>[6x]GMNKPCIISVAITGSLPRKKDNPAVPITVSEQVESTQAAFEAGATLVHLHVRNDDETPTSNPDRFALVLEGIRKHAPGMITQVSTGGRSGAGNERGAMLSLRPDMASLATGSVNFPTRVYDNPPELVDWLAAEMKTYGIKPEV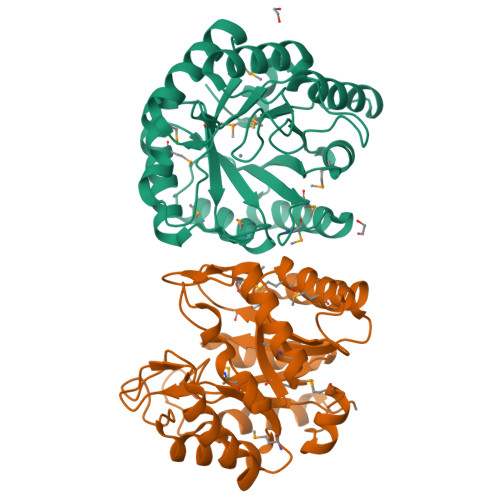EAFDLSMIFQAAAMQAAGAIVGPLHIQFVMGIKNAMPVDREVLEFYVQTLKRLSPDATWTGAGIGRHQLTMARWSLELGGHCRTGLEDNVRLDKNTLAPSNAALVRQVAELCEEYGRPVATAAQAREIMSLG> SFREQDIYLPIANVARIMKNAIPQTGKIAKDAKECVQECVSEF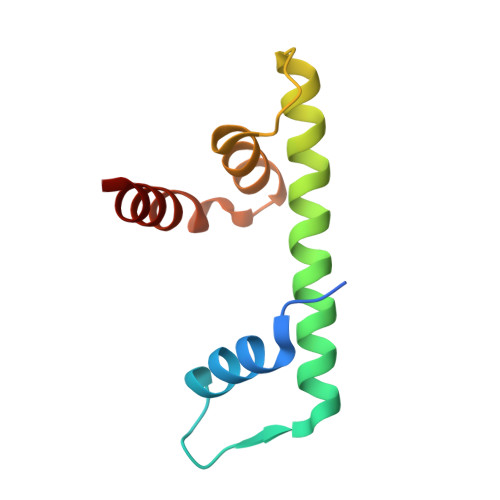ISFITSEASERCHQEKRKTINGEDILFAMSTLGFDSYVEPLKLYLQKFRE> MVSNWNWSGKKGRRTPRRGYTRPFKSAVPTTRVVVHQSAVLKKDDVSGSEIKPEGDVARYKIRKVMLSCTLRMRPGELVNYLIVKCSSPIVNWSAAFTAPALMVKES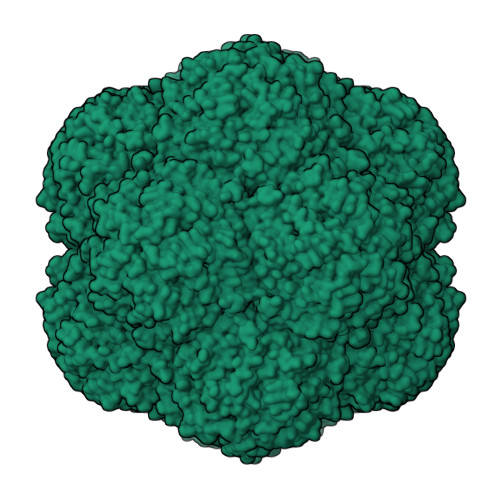CQDMITIIGKGKVESNGVAGSDCTKSFNKFIRLGAGISQTQHLYVVMYTSEAVKTVLEHRVYIEV>[8x]VPGPEYKVAILTVSDTVSAGAGPDRSGPRAVSVVDSSSEKLGGAKVVATAVVPDEVERIKDILQKWSDVD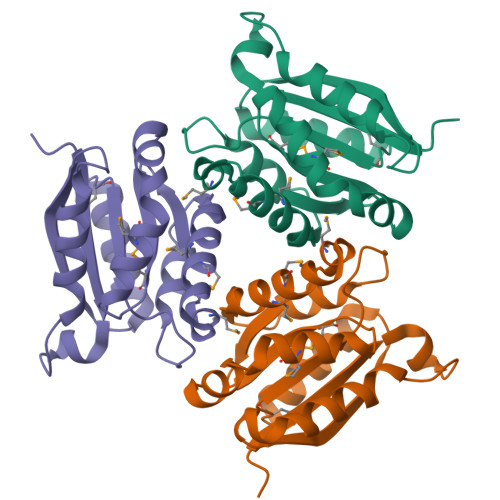EMDLILTLGGTGFTPRDVTPEATKKVIERETPGLLFVMMQESLKITPFAMLSRSAAGIRGSTLIINMPGNPNAVAECMEALLPALKHALKQI> E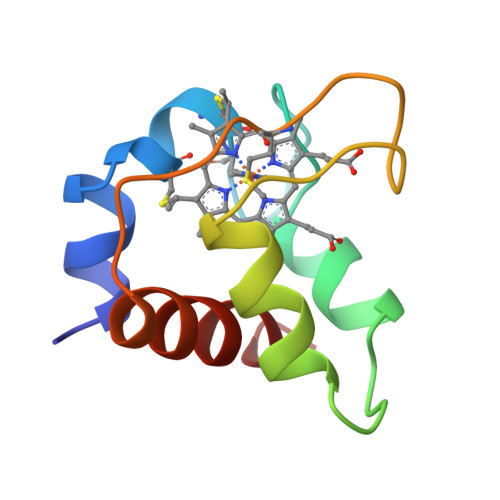DPEVLFKNKGCVACHAIDTKMVGPAYKDVAAKFAGQAGAEAELAQRIKNGSQGVWGPIPMPPNAVSDDEAQTLAKWVLSQK> MKYLLPTAAAGLLLLAAQPAMAMDSSGLEVLFQGPGSTSAQAPPVRRLPARFGVEQVRELASRDTRQGVGAGGIAWAISELDLAPVYLNFAENSHLMVTGRRECGRTTTLATIMSEIGRLYAPGASSAPPPAPGRPSAQVWLVDPRRQLLTALGSDYVERFAYNLDGVVAMMGELAAALAGREPPPGLSAEELLSRSWWSGPEIFLIVDDIQQLPPGFDSPLHKAVPFVNRAADVGLHVIVTRTFGGWSSAGSDPMLRALHQANAPLLVMDADPDEGFIRGKMKGGPLPRGRGLLMAEDTGVFVQVAATEVRRLEHH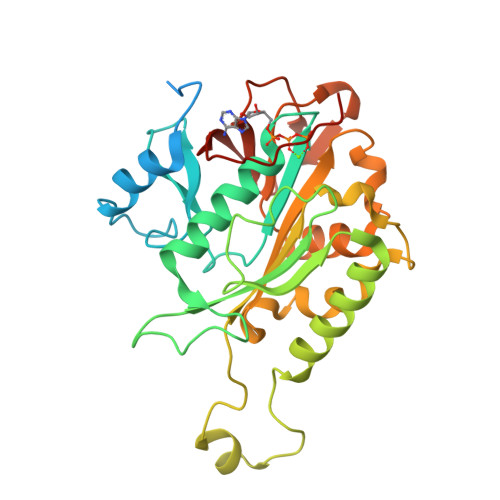HHHH> QLATKAARKSAPATGGV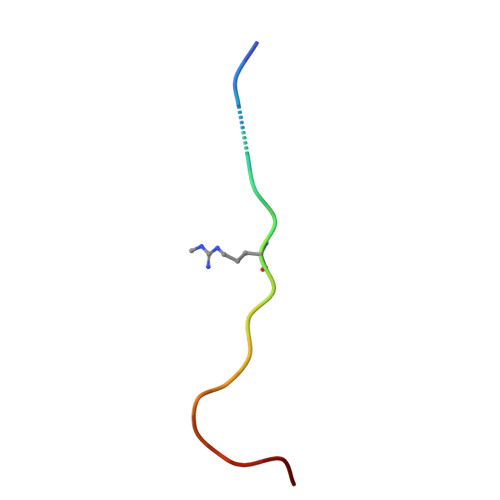K> ADTKEVLEAREAYFKSLGGSMKAMTGVAKAFDAEAAKVEAAKLEKILATDVAPLFPAGTSSTDLPGQTEAKAAIWANMDDFGAKGKAMHDAGGAVIAAANAGDGAAFGAALQKLGGTCK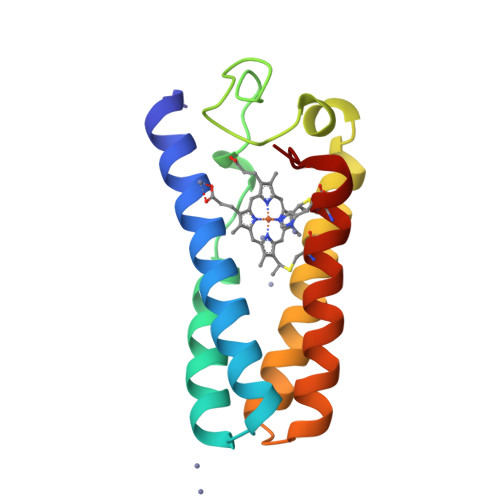ACHDDYREED>SMKLDIKKTFSNRSDRVKGIDFHPTEPWVLTTLYSGRVEIWNYETQVEVRSIQVTE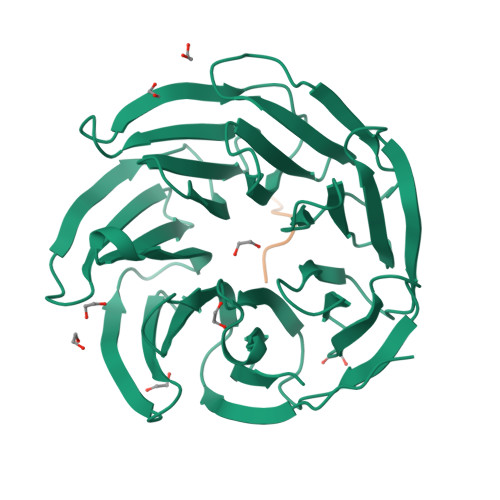TPVRAGKFIARKNWIIVGSDDFRIRVFNYNTGEKVVDFEAHPDYIRSIAVHPTKPYVLSGSDDLTVKLWNWENNWALEQTFEGHEHFVMCVAFNPKDPSTFASGCLDRTVKVWSLGQSTPNFTLTTGQERGVNYVDYYPLPDKPYMITASDDLTIKIWDYQTKSCVATLEGHMSNVSFAVFHPTLPIIISGSEDGTLKIWNSSTYKVEKTLNVGLERSWCIATHPTGRKNYIASGFDNGFTVLSLG[2x];>GVKLHYE[2x]> GMKTIDLADIQAFLYRESRLLDDKAWDAWLDCYRADAVFWMPSWDDADALVTDPQREISLIYYPNRQGLEDRVFRIKTERSSATVPDTRTSHNIANVERESADGDVHTVRFNWHTLSYRYKTVSSYFGMSRYAIDFSGDAPKIVSKYVVLKNDYINQ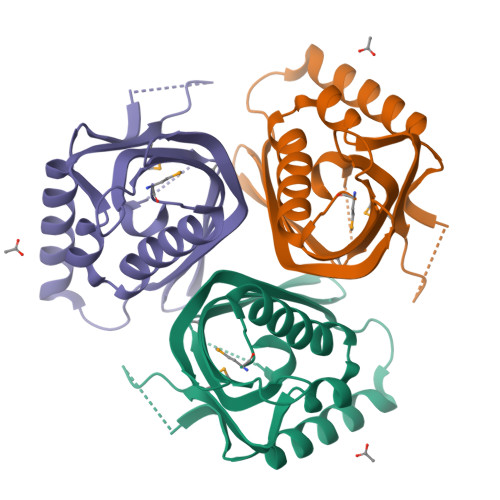LIDIYHI4'-(alpha-D-Mannopyranosyloxy)-biphenyl-4-methyl sulfonamide | C19 H23 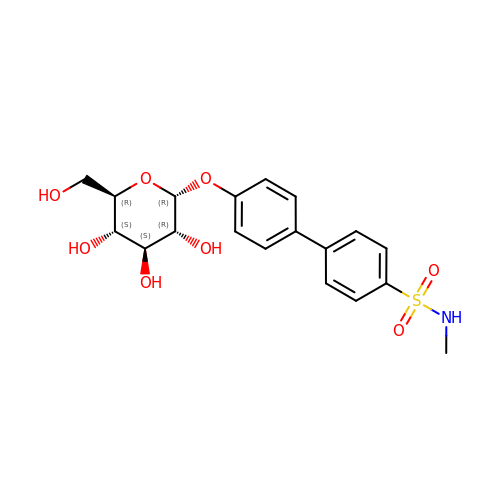N O8 S | CVQPQNFDTNLHAE-FQBWVUSXSA-N2'-deoxy-4'-ethynyl-2-fluoroadenosine 5'-(dihydrogen phosphate) | C12 H13 F N5 O6 P | 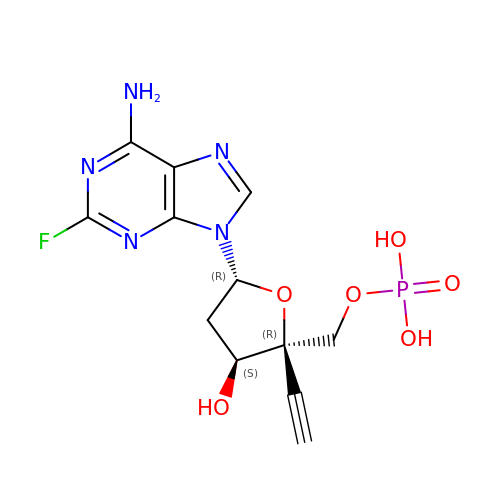MAIQRKKYFLNZMS-QRPMWFLTSA-N The biocatalytic reduction of the oxime moiety to the corresponding amine group has only recently been found to be a promiscuous activity of ene-reductases transforming α-oximo β-keto esters. By studying the crystal structures of enzyme oxime complexes, analyzing molecular dynamics simulations, and investigating biocatalytic cascades and possible intermediates, we obtained evidence that the reaction proceeds via an imine intermediate and not via the hydroxylamine intermediate. To gain more insight into the reaction pathway, we determined the crystal structures of the two enzymes OPR3 and XenA in complex with the oxime substrates 1a–c, either by co-crystallization or by soaking. All the crystal structures obtained had a high resolution (1.9–1.35 Å) and showed clear electron density features for the oximes.

In general, XenA structures showed a better-defined electron density for the substrate when prepared by soaking, while for OPR3, clearer results were obtained by co-crystallization. As an additional aspect of the crystallographic study, the structure of XenA with 1b might explain why only XenA efficiently transformed substrate 1b, and OPR3 did not. A closer look to the active site of XenA revealed a pocket delimited by the residues A57, I66, H178, H181, and Y183, which is not present in other previously investigated enzymes. Therefore, the presence of this pocket in XenA might explain why it is the only enzyme able to reduce oxime 1b efficiently and why oximes with substituents larger than an ethyl group are not accepted as substrates. Remarkably, a non-canonical tyrosine residue was found to contribute to the catalytic activity of the ene-reductase OPR3, protonating the hydroxyl group of the oxime in the first reduction step. Comparison with the other previously investigated enzymes revealed that this tyrosine is structurally conserved, though in class I/II OYEs, it is located close to the C-terminus of the enzyme (Y370 in OPR3). For OPR3, a non-canonical tyrosine residue was suggested as potentially catalytically relevant for the transformation of oxime substrates.

>[2x]HHHHHHMASSAQDGNNPLFSPYKMGKFNLSHRVVLAPMTRCRALNNIPQAALGEYYEQRATAGGFLITEGTMISPTSAGFPHVPGIFTKEQVREWKKIVDVVHAKGAVIFCQLWHVGRASHEVYQPAGAAPISSTEKPISNRWRILMPDGTHGIYPKPRAIGTYEISQVVEDYRRSALNAIEAGFDGIEIHGAHGYLIDQFLKDGINDRTDEYGGSLANRCKFITQVVQAVVSAIGADRVGVRVSPAIDHLDAMDSNPLSLGLAVVERLNKIQLHSGSKLAYLHVTQPRYVAYGQTEAGRLGSEEEEARLMRTLRNAYQGTFICSGGYTRELGIEAVAQGDADLVSYGRLFISNPDLVMRIKLNAPLNKYNRKTFYTQDPVVGYTDYPFLQGNGSNGPLSRL> GAASKKVNVLVVGLDNSGKTTIIERLKPRPRQAAEVAPTVGFTVDEVEKGPLTFTVFDMSGAGRYRTLWEQYYREADAVVFVVDSADKLRMVVARDEMEHMLKHSNMRKVPILYFANKKD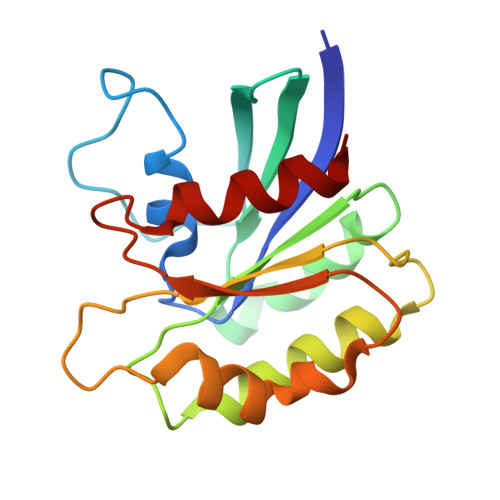IPVAMPPVEIAQALGLDDIKDRPWQIVPSNGLTGEGVDKGIDWLAERLS> NALPTWWKQAVFYQVYPRSFKDTNGDGIGDLNGIIENLDYLKKLGIDAIWINPHYDSPNTDNGYDIRDYRKIMKEYGTMEDFDRLISEMKKRNMRLMIDIVINHTSDQHAWFVQSKSGKNNPYRDYYFWRDGKDGHAPNNYPSFFGGSAWEKDDKSGQYYLHYFAKQQPDLNWDNPKVRQDLYDMLRFWLDKGVSGLRFDTVATYSKIPNFPDLSQQQLKNFAEEYTKGPKIHDYVNEMNREVLSHYDIATAGQIFGVPLDKSIKFFDRRRNELNIAFTFDLIRLDRDADERWRRKDWTLSQFRKIVDKVDQTAGEYGWNAFFLDNHDNPRAVSHFGDDRPQWREHAAKALATLTLTQRATPFIYQGSELGMTNYPFKKIDDFDDVEVKGFWQDYVETGKVKAEEFLQNVRQTSRDNSRTPFQWDASKNAGFTSGTPWLKINPNYKEINSADQINNPNSVFNYYRKLIN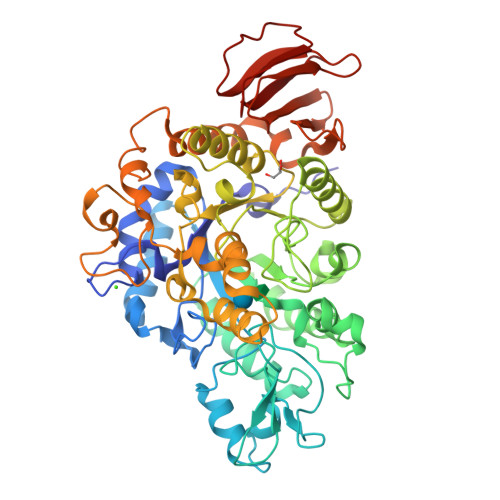IRHDIPALTYGSYIDLDPDNNSVYAYTRTLGAEKYLVVINFKEEVMHYTLPGDLSINKVITENNSHTIVNKNDRQLRLEPWQSGIYKLNP We have cloned a similar chitin deacetylase (EAA66447) from Aspergillus nidulans FGSC A4 and carried out an extensive characterization of the recombinant enzyme, with an appended short N-terminal His-tag, produced in E. coli. Combining mass spectrometry and analyses of acetate release, it was shown that AnCDA catalyses mono-deacetylation of (GlcNAc)2 and full deacetylation of (GlcNAc)3–6 in a non-processive manner. AnCDA seems to have broader substrate specificity than other characterized members of the CE4 family and the enzyme seems well suited to act on chitin and its partially deacetylated forms.

To characterize the nature of the substrate-binding site in AnCDA, we determined the crystal structure of the enzyme to 2.0 Å resolution. The structure shows the expected (β/α)8 barrel topology as well as a CE4 active site architecture, including the His-His-Asp metal-binding triad (H97, H101, D48), a catalytic acid (His196, aiding sugar departure) and a catalytic base (Asp47, activating the nucleophilic water), similar to the active site of ClCDA9. Despite the fact that no metals were added in the crystallization solution, there is clear evidence for a metal ion bound to the His-His-Asp triad, with a peak >14 σ in the 2Fo-Fc map. The ion, refined as cobalt, adopts an octahedral coordination in which the other three ligands are a bidentate phosphate molecule from the crystallization solvent and a water. The phosphate ion in AnCDA occupies the position where the acetyl-group of the to-be-deacetylated sugar, i.e. the sugar bound in subsite 0, is located. The sugar bound in subsite +1 interacts with Leu139 and Leu194 that form a hydrophobic pocket, similar as for ClCDA9. Interestingly, AnCDA (and ClCDA) have a lysine (Lys164 in AnCDA) within hydrogen-bonding distance to the sugar bound in subsite +1, creating a positively charged environment. This could reduce the affinity for deacetylated sugars in this subsite as the amino group of such a sugar carries positive charge. Another interesting feature of the AnCDA structure is the presence of a cluster of large aromatic residues on the surface of the protein near the catalytic centre and the −1 subsite. This cluster is composed of Tyr53, which is a phenylalanine in ClCDA and tyrosine in all three putative A. nidulans deacetylases, and Tyr200 and Trp201, which are unique to AnCDA.

>MAHHHHHHHRSTPLPLVRRVPTGQVITQCTTPNTIALTFDDGPSEYTPQLLDLLSRYSARATFFVLGDAAAQNPGLLQRMRDEGHQVGAHTYDHVSLPSLGYDGIASQMTRLEEVIRPALGVAPAYMRPPYLETNELVLQVMRDLDYRVISASVDTKDYENQDADAIINTSFQLFLDQLDAGGNIVLAHDIHYWTVASLAERMLQEVNARGLIATTVGDCLGDGEIAWYH[2x]>[2x]GARRFLCGVVEGFYGRPWVMEQRKELFRRLQKWELNTYLYAPKDDYKHRMFWREMYSVEEAEQLM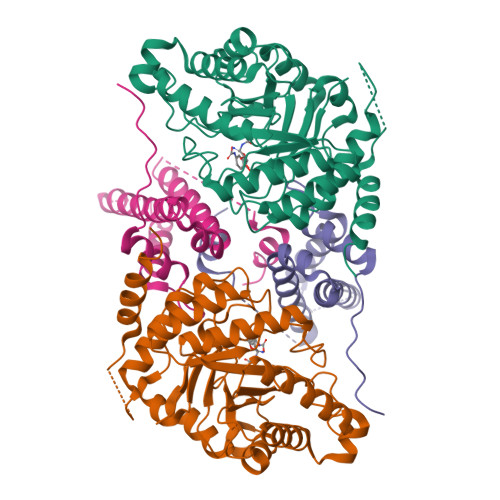TLISAAREYEIEFIYAISPGLDITFSNPKEVSTLKRKLDQVSQFGCRSFALLFDDIDHNMCAADKEVFSSFAHAQVSITNEIYQYLGEPETFLFCPTEYCGTFCYPNVSQSPYLRTVGEKLLPGIEVLWTGPKVVSKEIPVESIEEVSKIIKRAPVIWDNIHANDYDQKRLFLGPYKGRSTELIPRLKGVLTNPNCEFEANYVAIHTLATWYKSNMNGVRKDVVMTDSEDSTVSIQIKLENEGSDEDIETDVLYSPQMALKLALTEWLQEFGVPHQYSSR;>[2x]MEKPLYTAEPVTLEDLQLLADLFYLPYEHGPKGAQMLREFQWLRANSSVVSVNCKGKDSEKIEEWRSRAAKFEEMCGLVMGMFTRLSNCANRTILYDMYSYVWDIKSIMSMVKSFVQWLGCRSHSSAQFLIGDQEPWAFRGGLAGEFQRLLPIDGANDLFFQP>XQIARLQR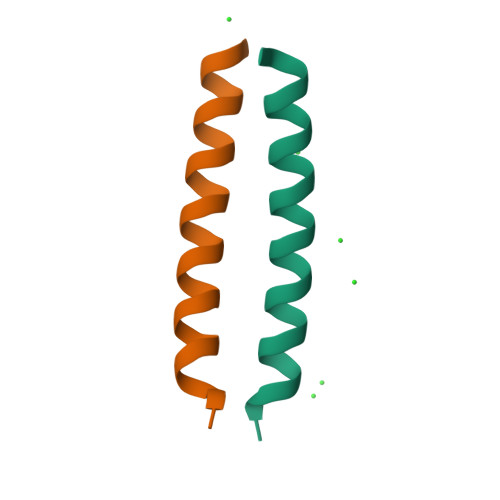QIRALQRQNARLQRQIRALQWX[2x]>[2x]DNILYSGETLSPGESLNYGPYTFIMQQDCNLVLYDVDK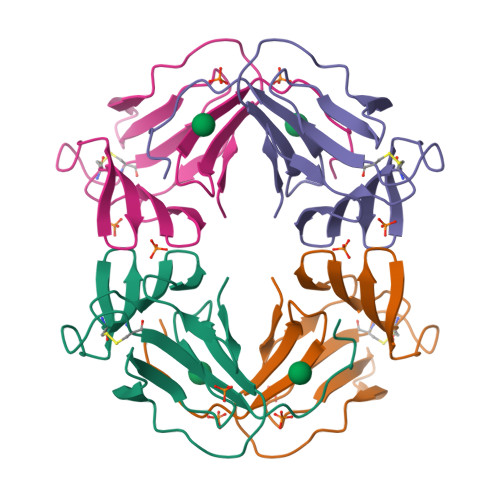PIWASNTGGLAQGCHLSMQSDGNLVVYSPSGNRIWASNTQGENGNYVCIVQKDRNVVIYGTARWATGTNI> IVVYTDREVYGAVGSQVTLHCSFWSSEWVSDDISFTWRYQPEGGRDAISIFHYAKGQPYIDEVGTFKERIQWVGDPSWKDGSIVIHNLDYSDNGTFTCD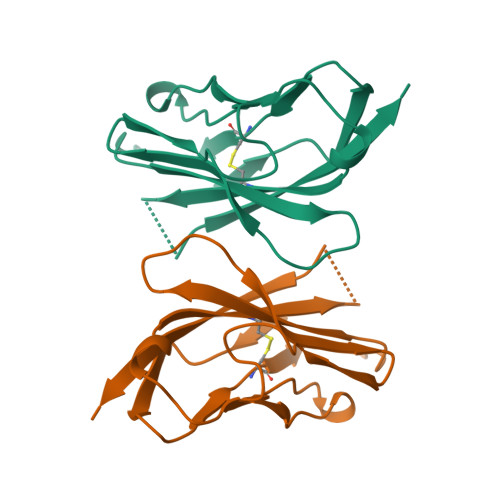VKNPPDIVGKTSQVTLYVFEKVPTR> GSKPLAEQDWYHGAIPRIEAQELLKKQGD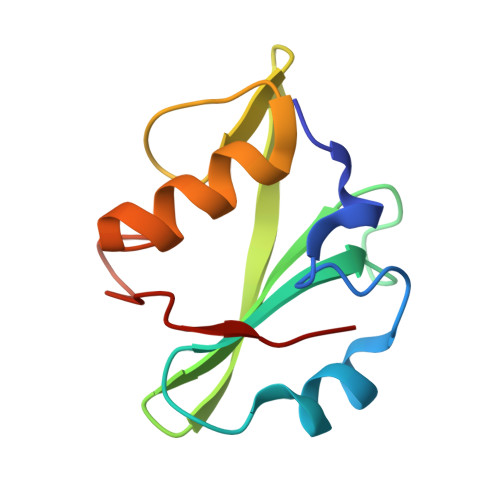FLVRESHGKPGEYVLSVYSDGQRRHFIIQYVDNMYRFEGTGFSNIPQLIDHHYTTKQVITKKSGVVLLNPIPK> MEFDDDLVDAEGNLVEQGGTYYLLPHIWAHGGGIETAKTGNEPCPLTVVRSPNEVSKGEPIRISSQFLSLFIPRGSLVALGFANPPSCAASPWWTVVDSPQGPAVKLSQQKLPE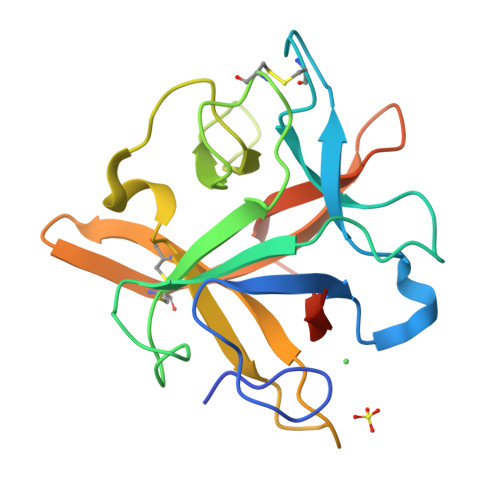KDILVFKFEKVSHSNIHVYKLLYCQHDEEDVKCDQYIGIHRDRNGNRRLVVTEENPLELVLLKAKSETASSH> MDETDPILTQKNWDGTATYFQSSDEHGFSMYYKPQVGFVGDPMPFYDPVAKDFKVMYLQDYRPNPEATYHPIFGVATKDGATYESLGELISCGGRDEQDAAIGTGGTIYNPADKLYYTFYTGNKFKPSSDQNAQVVMVATSPDFKTWTKNRTFYLKGDTYGYDKNDFRDPFLFQTEDGVYHMLIATRKNGKGHIAEFTSADLKEWESAGTFMTMMWDRFYACPDVFKMGDWWYLIYSEQASFMRKVQYFKGRTLEDLKATTANDAGIWPDNREGMLDSRAFYAGKTASDGTNRYIWGWCPTRAGNDNGNVGDVEPEWAGNLVAQRLIQHEDGTLTLGVPDAIDRKYTSAQEVKVMAKDGNMIESGKTYTLGEGASVIFNRLKVHNKISFTVKTASNTDRFGISFVRGTDSASWYSIHVNADEGKANFEKDGDDAKYLFDNKFNIPADNEYRVTIYSDQSVCVTYINDQLSFTNRIYQMQKNPWSLCCYKGEITVSDVQVSTYHHHHHH

Here we introduce the first crystal structures of the B. thetaiotaomicron endo-levanase BT1760 (EC 3.2.1.65). As typical for GH32 family enzymes, the BT1760 comprises an N-terminal five-bladed β-propeller catalytic domain and a tightly packed C-terminal β-sandwich module linked to it through a short helix. The distance between the nucleophile Asp41 and the general acid/base Glu221 in the structure of BT1760 is 5.2 Å suggesting double displacement mechanism of the endo-levanase reaction with retention of the configuration of the anomeric carbon atom. For BT1760, respective amino acids are Asp41, Asp169 and Glu221.

The E221A mutant was proved catalytically inactive: its catalytic activity towards levan (measured according to the reducing sugar release) was reduced by about 4,000 fold compared to the wild-type enzyme. A native dataset to 1.90-Å resolution was collected from a crystal that was soaked overnight with levantetraose (L-FOS, FFFF), a levan degradation intermediate that can be further cleaved by the endo-levanase. The ligand-bound structure of BT1760 revealed four subsites for the binding of fructose residues. According to sugar-binding subsite designation as recommended by, three ‘minus’ subsites and one ‘plus’ subsite were specified in the active site. The nucleophile Asp41 is located just below the fructose residue bound at −1 subsite, ready to attack the anomeric carbon (C2). No rotameric changes but only minor side chain shifts (up to 0.5 Å) were detected in the binding pocket compared to the wild-type structure model, thus substrate binding likely does not induce any major conformational changes. Since this carboxylic moiety is missing in the E221A mutant, the neighbouring Gln239 was found in two alternate conformations partially filling the artificial void. The levantetraose-bound structure of BT1760 shows that the −1 subsite accommodates a fructose residue that lies almost parallel to the bottom of the pocket defining the deepest-located (designated by us as level 0) binding subsite for a fructose residue. The levantetraose-bound structure of the E221A mutant of BT1760 suggests that the levan chain should be bent into the active site cavity to enable endo-cleavage. As the strongest proof for that we detected no levantetraose bound to this module in the crystallized protein – the only ligand molecule was found bound to the active site pocket of the catalytically inactive mutant of BT1760.>SMSDESVYKVLLLGAPGVGKSALARIFGGVEDGPEAEAAGHTYDRSIVVDGEEASLMVYDIWEQDGGRWLPGHCMAMGDAYVIVYSVTDKGSFEKASELRVQLRRARQTDDVPIILVGNKSDLVRSREVSVDEGRACAVVFDCKFIETSAALHHNVQALFEGVVRQIRLR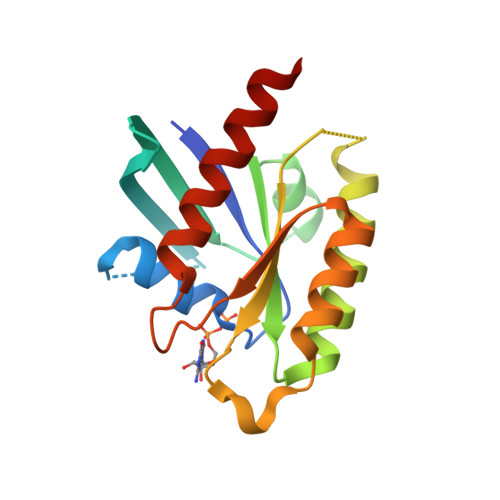RDSKEA[2x]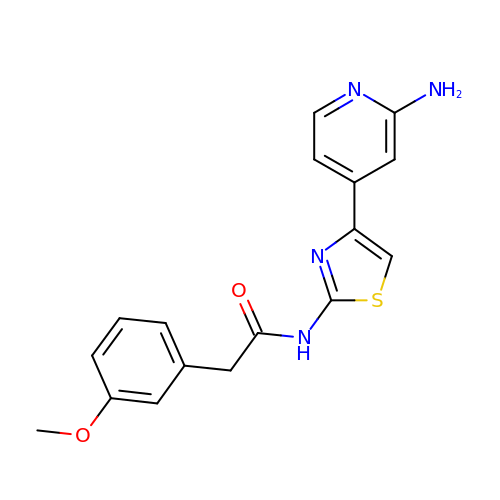N-[4-(2-aminopyridin-4-yl)-1,3-thiazol-2-yl]-2-(3-methoxyphenyl)acetamide | C17 H16 N4 O2 S | HIGGJLMBFDDVKA-UHFFFAOYSA-N>MKLVTVIIKPFKLEDVREALSSIGIQGLTVTEVKGFGRQKGHAELYRGAEYSVNFLPKVKIDVAIADDQLDEVIDIVSKAAYTGKIGDGKIFVAELQ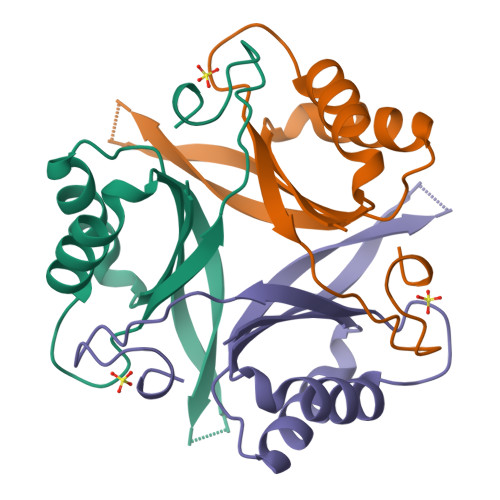RVIRIRTGEADEAAL[2x]> MGSMPYATQLALLQDELLDMLEPRDGEGLRTADIIDKTLRFRELLGCYRLQVEKSTRQLELPRQVRTA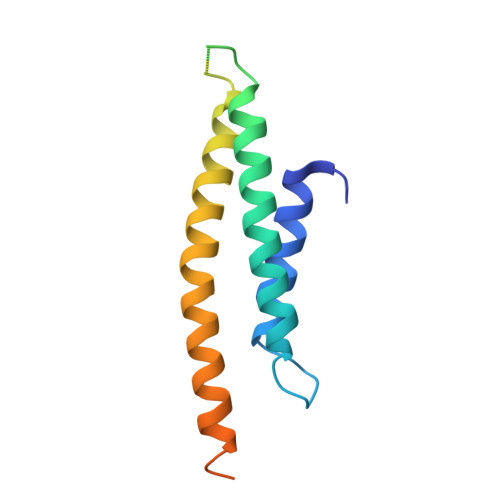AALRGAHAPASQAPALAQLLLWERFLADYRRRLDAAIVHEHEATAARQLQARPTAARAPRAPMTAKDRLLA> MPFRTIARLNPAKPKAGEEFRLQVVAQHPNEPGTRRDAEGKLIPAKYINLVEVYFEG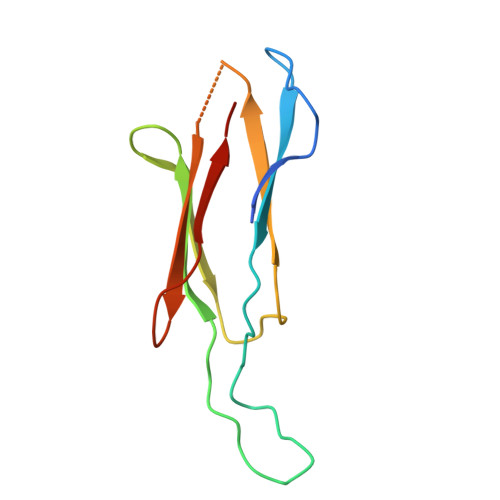EKVAEARPGPSTSANPLYAFKFKAEKAGTFTIKLKDTDGDTGEASVKLELA> MFSAGHKIKGTVVLMPKNELEVNPDGSAVDNLNAFLGRSVSLQLISATKADAHGKGKVGKDTFLEGINTSLPTLGAGESAFNIHFEWDGSMGIPGAFYIKNYMQVEFFLKSLTLEAISNQGTIRFVCNSWVYNTKLYKSVRIFFANHTYVPSETPAPLVEYREEELKSLRGNGTGERKEYDRIYDYDVYNDLGNPDKSEKLARPVLGGSSTFPYPRRGRTGRGPTVTDPNTEKQGEVFYVPRDENLGHLKSKDALEIGTKSLSQIVQPAFESAFDLKSTPIEFHSFQDVHDLYEGGIKLPRDVISTIIPLPVIKELYRTDGQHILKFPQPHVVQVSQSAWMTDEEFAREMIAGVNPCVIRGLEEFPPKSNLDPAIYGDQSSKITADSLDLDGYTMDEALGSRRLFMLDYHDIFMPYVRQINQLNSAKTYATRTILFLREDGTLKPVAIELSLPHSAGDLSAAVSQVVLPAKEGVESTIWLLAKAYVIVNDSCYHQLMSHWLNTHAAMEPFVIATHRHLSVLHPIYKLLTPHYRNNMNINALARQSLINANGIIETTFLPSKYSVEMSSAVYKNWVFTDQALPADLIKRGVAIKDPSTPHGVRLLIEDYPYAADGLEIWAAIKTWVQEYVPLYYARDDDVKNDSELQHWWKEAVEKGHGDLKDKPWWPKLQTLEDLVEVCLIIIWIASALHAAVNFGQYPYGGLIMNRPTASRRLLPEKGTPEYEEMINNHEKAYLRTITSKLPTLISLSVIEILSTHASDEVYLGQRD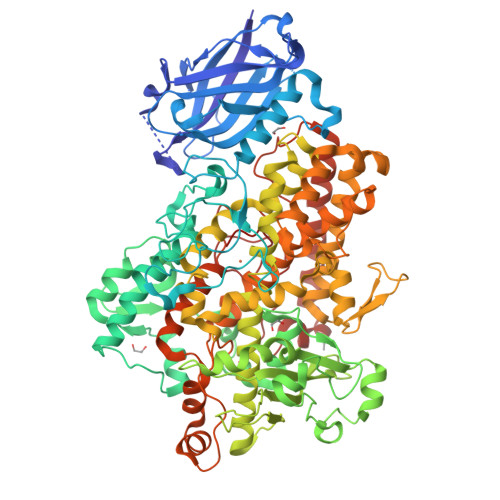NPHWTSDSKALQAFQKFGNKLKEIEEKLVRRNNDPSLQGNRLGPVQLPYTLLYPSSEEGLTFRGIPNSISI>MVKYPKQLFLESKNSKMNSIEMKYGQDPAINRAEFHVYGGVRQSKRKSEAWEAAKRITKERGIPNYNPDLHLKGAQMGQKVLQTYRITGLDREWAGGEDTPAHKGWKPGTDIAGLEMDDLNYENNPAMQQCYDDMRRTAINGLSIAHETIERRFGKEVTPETINLYFEMLNHNIGAGAIMMEHTAETNPELVKDSYAKCFTGNDELADALDQRFLIDINKMFPKYQADQIKAEVGDRIFQVARIPTMAVRTSDGGLSRAWVGQQASLAFLCAYDIPAGDAVTSDFVFTIKHGDVVFMGTQLPYRRAQRNNSAGGIALGYYSDCNQTSRTPEALEGLDGGIDPVKVIVEALTPGCVITDQGWLHNYLAGGSSGWSNYIISVYTDEVLEDYGYHGAIYAMDKWKCGVGEVPNTYENMMTIAEEVSRWSQKNYDEYPGLMEAHFGGSQRYSIQAAASGAAVGAMTGDPDLGNAAWHYNTPLCKEHYLRLGFYGHDLQDQQNMGHTYSYRSDQGIPYELKGPNYPDFAMNVGHMGGYIGIIAGAAHARGAAYSTNPIIKAAFADPNLQFDFRYPRREFGIGGLRQFMPAGERDAVIPPH[2x];>MAYLTEKIDLYGDNGKVLESDIPLEAVTPVQNPAVRELASIFKRSVAVNLGGAQKALSTGHYANEYIHFPDIPNKDKLGIKSSPGGKYPPKSVKVRTMDLPLVDDA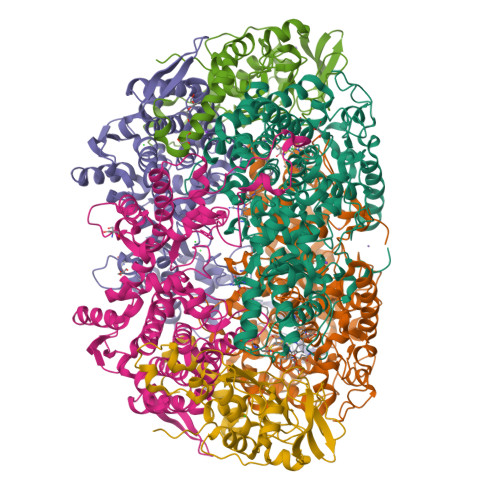DDIAARLKERLQVNPDDGTEVRVMKKGNVLYVKISEQLANTGVEYTTALTTTAQAMTDLVMEKYDLDFHASPLVHCAFYGRYPQTYEFMGGNVISLLAASCANEGPGFAMRNIMANHIVAATRKRTLEAVALSSTLEAIGHVEMGDAIGRWRRWQALVHACQGLNANNVVYDLVKEAGHGCTGDVVAATVGRALEDGIISVKKTLPSGYKFYTANDPSMWNAYVCAGLVAAVIVNQGAARAAQGVSSTLLYFNDLIEHETGLPHAGYGDGMGNGVSFSFFSHAIYGGGSPGIFSGNHIVTRHSKGFAIPVIAAAVSLDSGTAVYGPEATSGLVGDIFGEVDLIRRPMEAIASAAAEIKDKF[2x];>MVYQRQFLPADDRVTKNRKKVVDPSVKLEKIRTLSDKDFLTLIGHRHLGEAYRSVNPPLAEIGEPEDPIRELVPPTEGAKAGDRVCTIIMTDSVYNPPIAHYTRAWMYHNRFRGIDNGVYSGRVTLEMRERDLEEACRTLFETEICDASRDQVRQYTCTGHSCRLDPDGMMFDPIERCIMSGGNVVYQKDSFGNPVDTPINMGKPLSEEELIERTVVYRTDRGEPMTREGDPGAPDEEVREALQWSRRIQWLRMLGNMVPDKIKGM[2x]>SPGMELQVSSGFVCNTCPEKWINFQRKCYYFGKGTKQWVHARYAC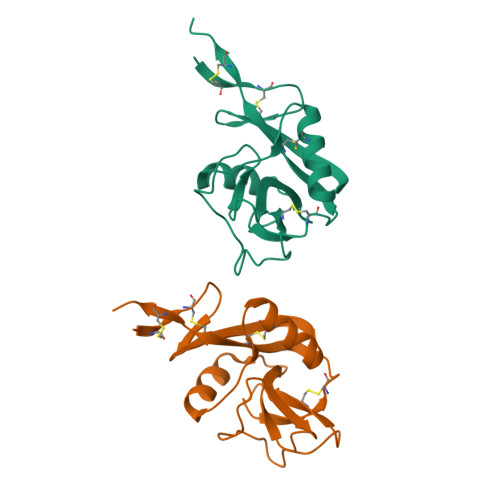DDMEGQLVSIHSPEEQDFLTKRASHTGSWIGLRNLDLKGEFIWVDGSHVDYSNWAPGEPTSRSQSEDCVMMRGSGRWNDAFCDRKLGAWVCDRLATCTPPASEGSAESMGPDSRPDPDGRLPTPSAPLHS[2x]>MTATDNARQVTIIGAGLAGTLVARLLARNGWQVNLFERRPDPRIETGARGRSINLALAERGAHALRLAGLEREVLAEAVMMRGRMVHVPGTPPNLQPYGRDDSEVIWSINRDRLNRILLDGAEAAGASIHFNLGLDSVDFARQRLTLSNVSGERLEKRFHLLIGADGCNSAVRQAMASVVDLGEHLETQPHGYKELQITPEASAQFNLEPNALHIWPHGDYMCIALPNLDRSFTVTLFLHHQSPAAQPASPSFAQLVDGHAARRFFQRQFPDLSPMLDSLEQDFEHHPTGKLATLRLTTWHVGGQAVLLGDAAHPMVPFHGQGMNCALEDAVALAEHLQSAADNASALAAFTAQRQPDA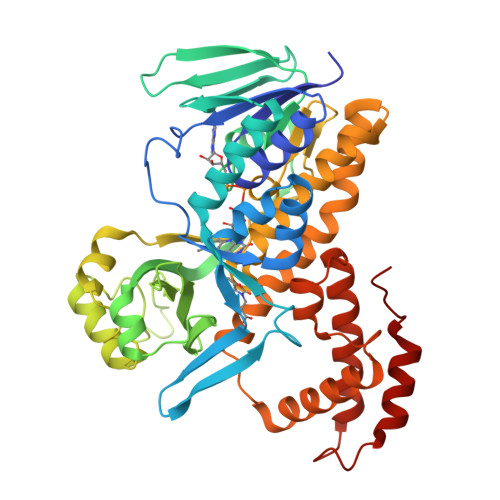LAIQAMALENYVEMSSKVASPTYLLERELGQIMAQRQPTRFIPRYSMVTFSRLPYAQAMARGQIQEQLLKFAVANHSDLTSINLDAVEHEVTRCLPPLSHLS[4x]> MRGSHHHHHHGSELSQEVTQTLKQWRVAAVSSAGLKYYVGVDIGGTNTRLALARAEDHDTFLQVLKVKADDTRKLIAFFDSVSDSIRDLLGVEASGACLAGAGRISPDGEVLDVTNFHGDATHRRLKRSELPSFLFPPTKTHFINDLEGTCYGVSSMNASDALDQCFKPLWGPASSDKVTLQPDHYLVLAVGTGLGIATLLSLRRSPVRGGFQVMPMEFGHVAISPVGPANAAYAEETRLLEYISEKLYNKEHAIEYEDIVSGRGLVITYKWVLDEANVQDESLRSLDAGKIAKNATNSEACPYAHKAMMLHF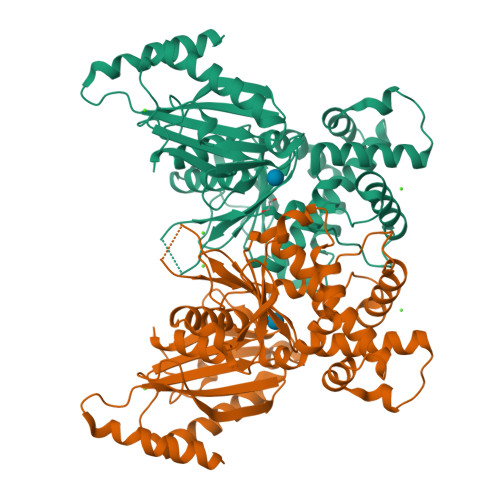KFLMRIAKNLCIGLQVRGMLLAGDNQVNNNLFLEQNLESLRAEFFDHPKKAWIEDIDLFTQTKPVNLNLHGALYVARG>[4x]MLRHLAGASALALTLAGAGFAQDHDHDHEDVTLYRVFVGDHEKGQVTAFDLAEPDHRWTFPTTGQVKLYSVAGGAVVAAVQSDADTVQFIRSGISFHDHGDHRDIEVGDPAAIDASLTGPRPFHLVEHDGKVVLNYDQGGYAEILDGHALAEGKAEPGRFPQARAHHGFVAPLGGNWLSTVASDEKVEGDASVPRLGLQAFDAEGNPAGNLATCTGIHGEAFSGAYLAAGCKEGVLTVKAGANGSEYKLLPYPADLPQGVTTGTLLGSTGIQVFLGNYGPDGLVVIDPVDEPHYRYIKLPFRRVDFALDPAKPSTGYVLTEDGSLHRIDLLKAEIVASAKVTEPYSMDGHWNDPRPRIAMAGDEIVVTDPNAGLVRRIATEDLSERGTVPVEGKPYNIAVTGGSGVTH

We have recently identified a periplasmic protein AztD in Paracoccus denitrificans, which is able to transfer zinc to the cluster A-I SBP AztC23. Here, we describe crystal structures of AztD homologs from P. denitrificans (PdAztD) and Citrobacter koseri (CkAztD), a pathogen of the carbapenem-resistant Enterobacteriacea group. In each case, the protein adopts a beta-propeller fold composed of continuous antiparallel beta sheets forming 8, 3-, and 4-stranded blades and containing a disulfide bond between highly conserved Cys214 and Cys231 (P. denitrificans numbering). Two high-affinity zinc-binding sites are identified, only one of which is competent for transfer to AztC.

The crystal structure of CkAztD has two monomers in the asymmetric unit while PdAztD has 4. Site 1 is present in the central pore of the protein and zinc is coordinated by His124, His167, His218, and a solvent molecule. Site 2 is contained on an extension from the body of the protein composed of the N- and C-terminal beta strands and a beta hairpin from blade 2. Zinc is coordinated by His99, His102, Asp104, and the side chain of the C-terminal His408. Zinc ligands at both sites are highly conserved in ≥95% of AztD homologues with the exception of His408, which is only conserved in 68.1% of analyzed sequences. All zinc occupancies refined to > 0.7 in PdAztD and 0.4 in CkAztD. The crystal structures do not allow us to determine whether associative transfer of zinc to AztC occurs from PdAztD site 1, site 2 or both. The mutagenesis data clearly demonstrates that zinc is transferred exclusively from AztD site 2 to AztC, leaving one to question the function of the highly conserved site 1. The cooperative nature of binding between sites 1 and 2 suggest that site 1 may function to tune the overall zinc-binding affinity to the needs of the organism.> MRLDQRWLIARVI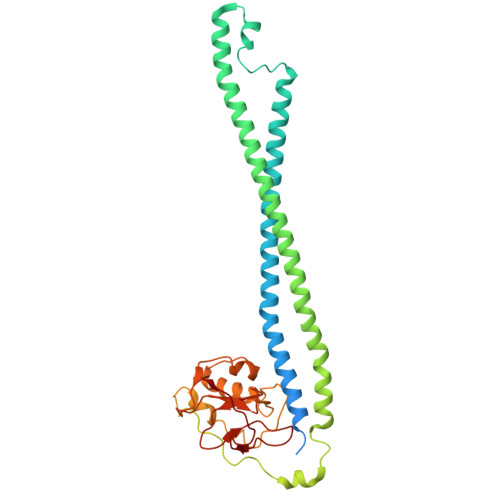MRSAIGFFASFTVSSGVLAANVLADPADDALAKLNELSRQAEQTTEALHSAQLDLNEKLAAQRAADQKLADNRTALDAARARLATFQTAVNKVAAATYMGGRTHGMDAILTAESPQLLIDRLSVQRVMAHQMSTQMARFKAAGEQAVKAEQAAAKSAADARSAAEQAAAVRANLQHKQSQLQVQIAVVKSQYVALTPEERTALADPGPVPAVAAIAPGAPPAALPPGAPPGDGPAPGVAPPPGGMPGLPFVQPDGAGGDRTAVVQAALTQVGAPYAWGGAAPGGFDCSGLVMWAFQQAGIALPHSSQALAHGGQPVALSDLQPGDVLTFYSDASHAGIYIGDGLMVHSSTYGVPVRVVPMDSSGPIYDARRY>[2x]GSWTKEEEEALLDGLDLVKGPRWSQILELYGPGGKKSEVLKYRNQVQLKDKAR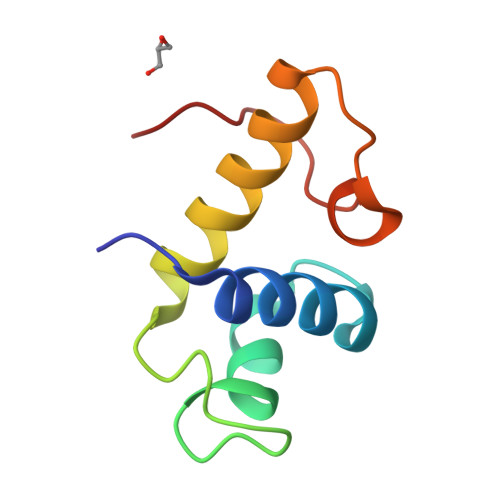NMKLFFLKSGQVVPAALQCVTGDLRRD> GSKWKVFIDQINRSLENYEPCSSQNCSCYHGVIEEDLTPFRGGISRKMMAEVVRRKLGTHYQITKNRLYRENDCMFPSRCSGVEHFILEVIGRLPDMEMVINVRDYPQVPKWMEPAIPVFSFSKTSEYHDIMYPAWTFWEGGPAVWPIYPTGLGRWDLFREDLVRSAAQWPWKKKNSTAYFRGSRTSPERDPLILLSRKNPKLVDAEYTKNQAWKSMKDTLGKPAAKDVHLVDHCKYKYLFNFRGVAASFRFKHLFLCGSLVFHVGDEWLEFFYPQLKPWVHYIPVKTDLSNVQELLQFVKANDDVAQEIAERGSQFIRNHLQMDDITCYWENLLSEYSKFLSYNVTRRKGYDQIIP;> GSDVNECVTNPCQNDATCLDQIGEFQCICMPGYEGVHCEVNT

POGLUT1 is an inverting GT-B fold (CAZy GT Family 9018) glycosyltransferase and its EGF-like domain substrates sit in a cleft formed between the canonical N-terminal and C-terminal domains. Here we report the structure of human POGLUT1 in complexes with three different EGF-like domains and either UDP, a donor substrate analog or a slow substrate. The structures reveal the basis for POGLUT1’s ability to recognize diverse EGF-like domain substrates and for the requirement that they be folded. The three EGF-like domains studied are positioned almost identically in their respective complexes and 25–30% of their surface (740–830 Å2) is buried by POGLUT1.

Unlike other protein-O-glycosyltransferases that can glycosylate both serine and threonine, POGLUT1 can only glycosylate serine3, 15, 27 and our structures now provide an explanation for why this is the case. The hydrogen bond to the POGLUT1 catalytic base, Asp133, fixes the serine hydroxyl of the acceptor substrate in the gauche (−) rotamer (χ1 = −70°) where it is aligned for nucleophilic attack. Given its main chain conformation (Φ = −90 ± 5°, Ψ = 15 ± 5°), threonine could not access this rotamer owing to the steric clash that would ensue between its sidechain methyl group and its own carbonyl oxygen atom. To confirm this rationalization, we mutated the O-glucosylation site of hEGF12 to a threonine residue (hEGF12:S458T) and measured its ability to be glucosylated and determined its structure in complex with POGLUT1 and UDP. Consistent with the requirement for serine, the threonine mutant was not glucosylated, even at a concentration of 100 μM, and as shown by the structure, the conformation of the O-glucosylation motif was essentially unchanged. However, the threonine sidechain was found in the gauche (+) conformation (χ1 = 66°) where it hydrogen bonds to Arg107 of POGLUT1 and the carbonyl oxygen atom of the C1(−1) residue of hEGF12. In this rotamer, the threonine hydroxyl group is not positioned for in-line nucleophilic attack and its methyl group makes contact with the sidechain of Asp133, an interaction that shifts the Asp carboxyl group relative to that seen in all of the other complexes. Contrary to that previously suggested, we now show that the serine specificity is a result of well-established mainchain–sidechain steric constraints. Given the mainchain conformation of the O-glucosylation motif, only serine can access the sidechain rotamer required for activation and in-line nucleophilic attack on C1 of the donor substrate.The eukaryotic pyruvate dehydrogenase complex (PDHc), as the most studied family member, is composed of multiple copies of the E1, E2, E3BP (also known as protein X), and E3 enzymes, which all work in concert to perform the dedicated pyruvate oxidation reaction. Architecturally, the core consists of 60 subunits that form a near-symmetric icosahedral structure, formed by 20 trimeric subunits at each corner. In fungi, the core-forming subunit is exclusively E218, whereas in mammals the core is composed of a mixture of E2 and E3BP in either a 48:1219 or 40:20 E2:E3BP ratio. The E2 active site binds CoA and catalyzes the transacetylase reaction, in which the acetyl group from the N6-lipoyllysine, located in the peripheral LD of E2 and E3BP, is transferred onto the thiol group of CoA.

Here, we report a cryo-EM structure of the fully active Chaetomium thermophilum pyruvate dehydrogenase complex (PDHc) core scaffold at 3.85 Å resolution (FSC = 0.143) from native cell extracts. The reconstruction of the core with an application of icosahedral symmetry was resolved at 3.85 Å resolution (FSC = 0.143), where the backbone is clearly traceable and side chain resolution is often visible. The overall icosahedral core is stabilized by two interfaces with distinct energetic signatures, which were calculated with HADDOCK. In particular, the intra-trimeric interface, buries a large surface area of ~5000 Å², while the inter-trimeric interface buries only ~1500 Å2. Inside this cavity, three arginines with a modeled distance of 3.26 Å are visible. We cannot rule out, that this close proximity is a result of averaging, but we suspect the existence of an arginine cluster. Another structural feature is a loop element facing inside the core cavity formed by residues Val405-Trp420, and maybe potentially critical for the organization of the PDHc core scaffold. Flexible regions were first detected above the E2 active site. A previously described backfolded structural element is not seen in the native PDHc core scaffold structure, allowing increased accessibility to the LD to be accommodated in the E2 active site.

> MLAQVLRRQALQHVRLARAAAPSLTRWYASYPPHTIVKMPALSPTMTSGNIGAWQKKPGDAITPGEVLVEIETDKAQMDFEFQEEGVLAKILKETGEKDVAVGSPIAVLVEEGTDINAFQNFTLEDAGGDAAAPAAPAKEELAKAETAPTPASTSAPEPEETTSTGKLEPALDREPNVSFAAKKLAHELDVPLKALKGTGPGGKITEEDVKKAASAPAAAAAAPGAAYQDIPISNMRKTIATRLKESVSENPHFFVTSELSVSKLLKLRQALNSSAEGRYKLSVNDFLIKAIAVACKRVPAVNSSWRDGVIRQFDTVDVSVAVATPTGLITPIVKGVEAKGLETISATVKELAKKARDGKLKPEDYQGGTISISNMGMNPAVERFTAIINPPQAAILAVGTTKKVAVPVENEDGTTGVEWDDQIVVTASFDHKVVDGAVGAEWMRELKKVVENPLELLL>MTSASSPPAFRLETSDGDEEGNAEVNKGKQEPPPMESPFQREDRNSSPQIKVNLNFIKRPPKNTSAPSQQEPDRFDRDRLFSVVSRGVPEELTGLLEYLRWNSKYLTDSAYTEGSTGKTCLMKAVLNLQDGVNACIMPLLQIDKDSGNPKLLVNAQCTDEFYQGHSALHIAIEKRSLQCVKLLVENGADVHLRACGRFFQKHQGTCFYFGELPLSLAACTKQWDVVTYLLENPHQPASLEATDSLGNTVLHALVMIADNSPENSALVIHMYDGLLQMGARLCPTVQLEEISNHQGLTPLKLAAKEGKIEIFRHILQREFSGPYQPLSRKFTEWCYGPVRVSLYDLSSVDSWEKNSVLEIIAFHCKSPNRHRMVVLEPLNKLLQEKWDRLVSRFFFNFACYLVYMFIFTVVAYHQPSLDQPAIPSSKATFGESMLLLGHILILLGGIYLLLGQLWYFWRRRLFIWISFMDSYFEILFLLQALLTVLSQVLRFMETEWYLPLLVLSLVLGWLNLLYYTRGFQHTGIYSVMIQKVILRDLLRFLLVYLVFLFGFAVALVSLSREARSPKAPEDNNSTVTEQPTVGQEEEPAPYRSILDASLELFKFTIGMGELA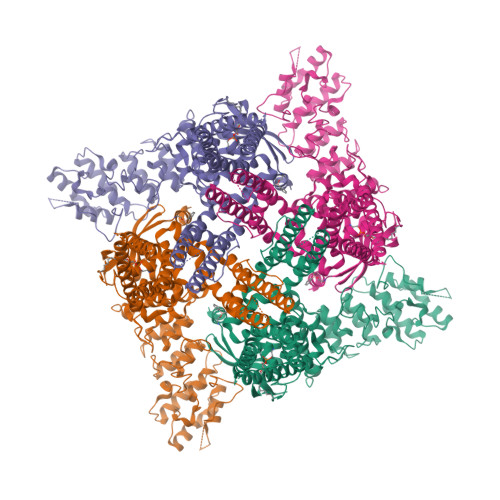FQEQLRFRGVVLLLLLAYVLLTYVLLLNMLIALMSETVNHVADNSWSIWKLQKAISVLEMENGYWWCRRKKHREGRLLKVGTRGDGTPDERWCFRVEEVNWAAWEKTLPTLSAAPSGPGITGNKKNPTSKPGKNSASEEDHLPLQVLQSP[4x]>[4x]MVVKVGVIGTGAMGRAHIDRLTNVLTGAEVVAVTDIDHEAAEAAVRDFHLNAKVYPDDTSLLQDPDIDAVFVVSFGGAHEATVLKALDTDKFIFTEKPLATTLEGAKRIVDKELTKSKKVIQVGFMRRYDQGIRALKEKLDTGIIGAPLVVRASHINPNVASNYSNEMAITDTLIHEIDEMHWLLDDEYTSIQITYPRQSAEVRNEGLHDPQLATLTTKKGTVIQVLVHVTAQYGYE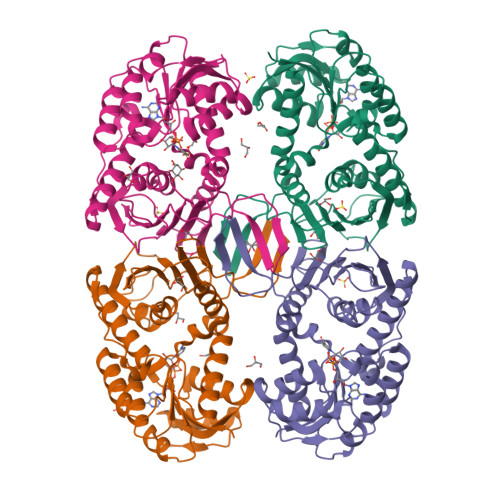VKLEVIGETGELQLPNYGLGPILRSNANQQTAVEMSWINRFIQAYNTEVQEFIDEVAKSEPPVGPSAWDGYIAAITAAAANRSQKDQETVLINVAGTPTFYQ> AKHTLLRHEGIETVSYATQSLVVANGGLGNGVSRNQLLPVLEKCGLVDALLMPPNKPYSFARYRTTEESKRAYVTLNGK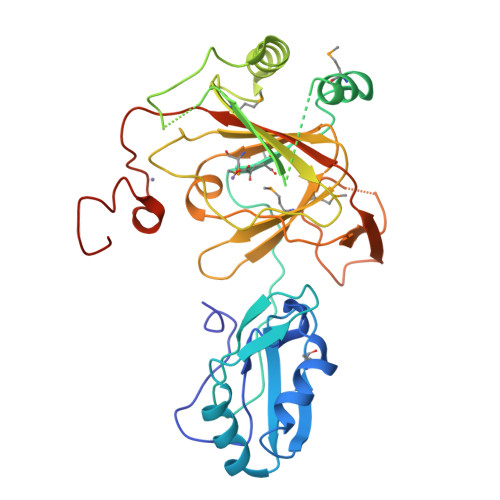EVVDDLGQKITLYLNFVEKVQWKELRPQALPPGLMVVEEIISSEEEKMLLESVDWTEDTDNQNSQKSLKHRRVKHFGYEFHYENNNVDKDKPLSGGLPDICESFLEKWLRKGYIKHKPDQMTINQYEPGQGIPAHIDTHSAFEDEIVSLSLGSEIVMDFKHPDGIAVPVMLPRRSLLVMTGESRYLWTHGITCRKFDTVQASESLKSGIITSDVGDLTLSKRGLRTSFTFRKVRQTPCNCSYPLVCDSQRKENLYFQGLEHHHHHH> RFILEISGDLACFTRSELKVERVSYPVITPSAARNILMAILWKPAIRWKVLKIEILKPIQWTNIRRNEVGTKMSERSGSLYIEDNRQQRASMLLKDVAYRIHADFDMTSEAGESDNYVKFAEMFKRRAKKGQYFHQPYLGCREFPCDFRLLEKAEDGLPLED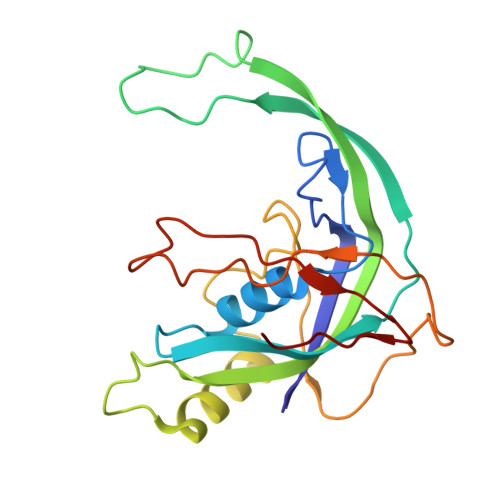ITQDFGFMLYDMDFSKSDPRDSNNAEPMFYQCKAVNGVITVPP>[2x]ENLKDEILEKYIPKTKKTRSGHIVIKTEETPNPEIVANTRTVPGIITARGCAYAGCKGVVMGPIKDMVHITHGPIGCSFYTWGGRRFKSKPENGTGLNFNEYVFSTDMQESDIVFGGVNKLKDAIHEAYEMFHPAAIGVYATCPVGLIGDDILAVAATASKEIGIPVHAFSCEGYKGVSQSAGHHIANNTVMTDIIGKGNKEQKKYSINVLGEYNIGGDAWEMDRVLEKIGYHVNATLTGDATYEKVQNADKADLNLVQCHRSINYIAEMMETKYGIPWIKCNFIGVDGIVETLRDMAKCFDDPELTKR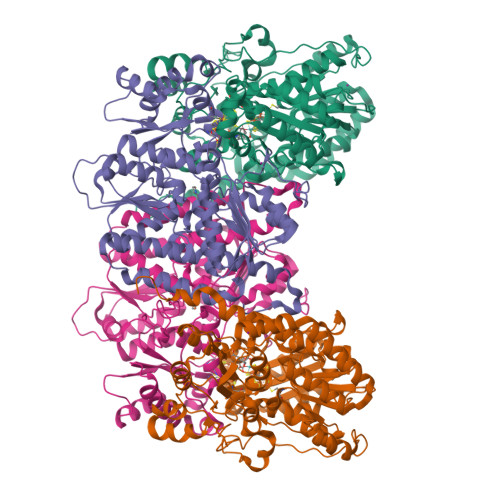TEEVIAEEIAAIQDDLDYFKEKLQGKTACLYVGGSRSHTYMNMLKSFGVDSLVAGFEFAHRDDYEGREVIPTIKIDADSKNIPEITVTPDEQKYRVVIPEDKVEELKKAGVPLSSYGGMMKEMHDGTILIDDMNHHDMEVVLEKLKPDMFFAGIKEKFVIQKGGVLSKQLHSYDYNGPYAGFRGVVNFGHELVNGIYTPAWKMITPPWK;>[2x]MLDATPKEIVERKALRINPAKTCQPVGAMYAALGIHNCLPHSHGSQGCCSYHRTVLSRHFKEPAMASTSSFTEGASVFGGGSNIKTAVKNIFSLYNPDIIAVHTTCLSETLGDDLPTYISQMEDAGSIPEGKLVIHTNTPSYVGSHVTGFANMVQGIVNYLSENTGAKNGKINVIPGFVGPADMREIKRLFEAMDIPYIMFPDTSGVLDGPTTGEYKMYPEGGTKIEDLKDTGNSDLTLSLGSYASDLGAKTLEKKCKVPFKTLRTPIGVSATDEFIMALSEATGKEVPASIEEERGQLIDLMIDAQQYLQGKKVALLGDPDEIIALSKFIIELGAIPKYVVTGTPGMKFQKEIDAMLAEAGIEGSKVKVEGDFFDVHQWIKNEGVDLLISNTYGKFIAREENIPFVRFGFPIMDRYGHYYNPKVGYKGAIRLVEEITNVILDKIERECTEEDFEVVR>MMEAMVKYLAEKAGISEVEAAEIVLKAVKISGGDVVKSIELVDLFIEILNKGR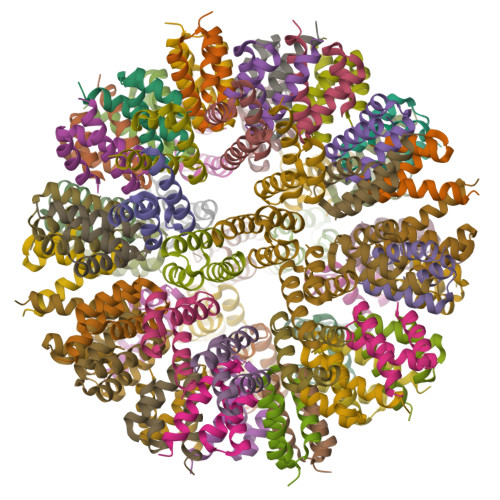E[60x]>[2x]MEFIMKTRMFEEEGWIRKKCKVCGKPFWTLDPDRETCGDPPCDEYQFIGKPGIPRKYTLDEMREKFLRFFEKHEIYPHGRVKRYPVLPRWRDDVLLVGASIMDFQPWVISGEADPPANPLVISQPSIRFTDIDNVGITGRHFTIFEMMAHHAFNYPGKPIYWMDETVELAFEFFTKELKMKPEDITFKENPWAGGGNAGPAFEVLYRGLEVATLVFMQYKKAPENA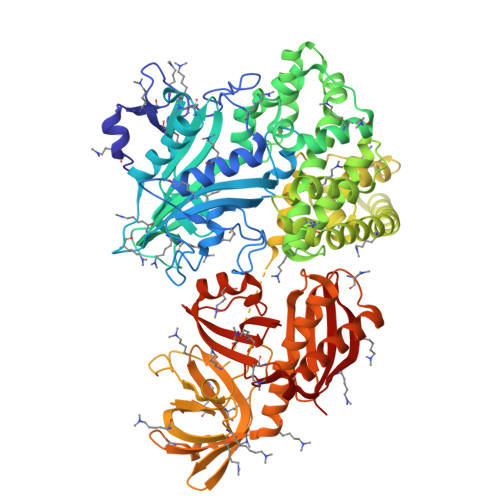PQDQVVVIKGEKYIPMETKVVDTGYGLERLVWMSQGTPTAYDAVLGYVVEPLKKMAGIEKIDEKILMENSRLAGMFDIEDLGDLRYLREQVAKRVGITVEELEKAIRPYELIYAIADHTKALTFMLADGVVPSNVKAGYLARLLIRKSIRHLRELGLEVPLSEIVALHIKELHKTFPEFKEMEDIILEMIELEEKKYAETLRRGSDLVRREIAKLKKKGIKEIPVEKLVTFYESHGLTPEIVKEIAEKEGVKVNIPDNFYSMVAKEAERTKEEKGEELVDFELLKDLPDTRRLYYEDPFMKEFDAKVLRVIKDWVILDATAFYPEGGGQPYDTGVLIVNGREVKVTNVQKVGKVIIHKVEDPGAFKEGMIVHGKIDWKRRIQHMRHHTGTHVLMGALVRVLGRHVWQAGSQLTTDWARLDISHYKRISEEELKEIEMLANRIVMEDRKVTWEWLPRTTAEQKYGFRLYQGGVVPGREIRVVKIEDWDVQACGGTHLPSTGLVGPIKILRTERIQDGVERIIFACGE> MGVRLYSCDACPHAVFTTHAALLAHAEEHHADLLPDHARLRRIAQKLNPVWNRALNARRNTITSWGKKIFHVAAQRDAGESKMQEAHRARAQLECVVRRWHDKARVFIFGSSVAMGVWDGTADIDFAVVDVDAMERGSWPPLEKNAVRSITELLRRVGFSFVNLEPISHARVPIIKHHASSPILTVARRDAEDVVARSIRFILNGPATREDRLLLEGSVRDAVGPTGVQQVWWNRTSDMMSATLESTTAA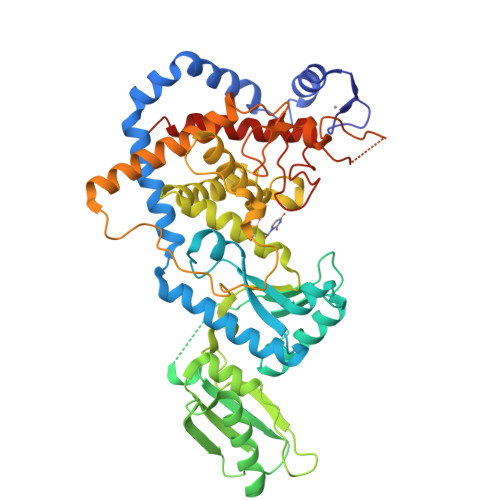VRAAMCSPALASASLRTKVQPAHDECRPELYNIDFALSFRAFGIRNSTLLRKYLLSHPCARPGAIVLKDWSKTSGVNNSVNGYFTSYAINIMWIYYLVQKGYVPYVDPLEIPESLVNYTDFDPRYTPMIDPEITNTEREELYKAAGDMLVGFFYFYSFEFDWGHNVISLNRPGITTKRMLGWHVEDVVPVASTSVSSGGGGSNVKRHPTRYELCIEDPYEENLNLGRHIGVTKSLRVRTELYRGLLSLLKEGETRSCVFAAA> MSTLFPKYSKTTDGSKVIMEQRLLQQVNNLILDNDICTGCGICSEVCPEEAISVGAVGGVRRGLV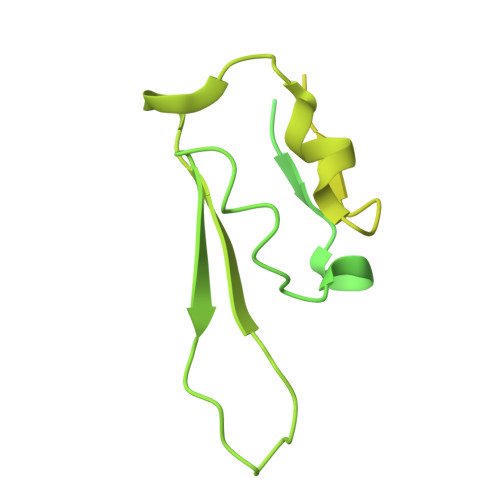DDAASIHVDETKCSYCGVCVIMCPFSALALKVDGEERLPILEKEGFPTYDKGTAIDQDKCVRCNICDDVCPRDAIDRDVPLFEGEDKEGLAKGQAVELKIEFKVDDEKCTKCGICGNLCEAINVLHKPFSPEIGKVEGEVIWDEAYCDGCNVCAEACPSEAIKVTRTVVGQKKLGNVNIIDEDCCTCRWCAINCPTEAITVNKIFEGEITFHAEKCPGGCSTCVDVCPANAIYLPTPKPAKDMKGQIEAKIAVNKDFCILCGACVNACPGEDIIYLRRDSVKIKGKETDLFKKIKEKLFTPRTSKVKEQPSLAGSVELKAVSQ Canonical human TFIID consists of TBP and 13 TBP-associated factors (TAFs). Among these HFD pairs, the TAF8–10 heterodimer plays a key role in the TFIID assembly pathway, is critical for the integrity of holo–TFIID and also fulfills essential functions in early embryonic development682627. By immunoprecipitating TAF-containing complexes from different cellular compartments, we identify a novel endogenous TFIID subcomplex formed by TAF2, 8 and 10 in the cytoplasm of human cells. Taken together, our data suggest the presence of a nuclear import particle in which the TAF2–8–10 complex is bound by the major binding site of Importin α1 via the NLS of TAF8, poised to shuttle into the nucleus.

A complex of TAF8–10 comprising TAF8 residues 25–120 and TAF10 residues 112–212 yielded crystals, which diffracted incident X-rays to 1.9 Å resolution. We determined the structure of this complex by the Sulfur-SAD method and refined the model to a crystallographic R value of 20.5% and a free R factor of 23.7% with excellent stereochemistry. The final model includes TAF8 residues 28–120 and TAF10 residues 113–212 with the exception of a flexible loop in TAF10 comprising residues 178–191. In our structure, TAF8 wraps entirely around the α2 helix of TAF10 markedly enveloping its interaction partner. Complex formation buries 2212.3 Å2 with predominantly hydrophobic intermolecular contacts. As observed in other HFD interactions, the two opposing aromatic residues Y68 of TAF8 and F162 of TAF10 at the crossover of the α2 helices contact each other via hydrophobic stacking interactions and categorize the complex to the H3/H4 family of HFD-containing proteins. The additional N-terminal α-helix of TAF10, αN and the C-terminal α-helix of TAF8, αC, contact each other on one side of the HFD in a head-to-tail fashion and significantly stabilize the complex by hydrophobic interactions centred on F119 of TAF10. In both proteins, a phenylalanine of loop L1 (F50 in TAF8 and F144 in TAF10) is embedded in a composite, hydrophobic cavity mainly formed by residues from helices α1/α2 of one protomer and helices α2/α3 of the other. The pseudosymmetric L1 loops are characteristic for the TAF8–10 complex, since similar arrangements cannot be found in the crystal structures of the Drosophila TAF6–TAF9 and the human TAF4–TAF12 complex2225 suggesting that the overall shape and precise geometry of the complex is important for integration into core–TFIID.

> GSSTPLVDFLMQLEDYTPTIPDAVTGYYLNRAGFEASDPRIIRLISLAAQKFISDIANDALQHCKMKGTASGSSRSKSKDRKYTLTMEDLTPALSEYGINVK;> MPADNYHLARRRTLQVVVSSLLTEAGFESAEKASVETLTEMLQSYISEIGRSAKSYCEHTARTQPTLSDIVVTLVEMGFNVDTLPAYAKRSQRMVIT>[4x]SRRTYTLTDYLKSTFRVKFYTLQWISDHEYLYKQENNILLFNAEYGNSSIFLENSTFDELGYSTNDYSVSPDRQFILFEYNYVKQWRHSYTASYDIYDLNKRQLITEERIPNNTQWITWSPVGHKLAYVWNNDIYVKNEPNLSSQRITWTGKENVIYNGVTDWVYEEEVFSAYSALWWSPNGTFLAYAQFNDTEVPLIEYSFYSDESLQYPKTVRIPYPKAGAENPTVKFFVVDTRTLSPNASVTSYQIVPPASVLIGDHYLCGVTWVTEERISLQWIRRAQNYSIIDICDYDESTGRWISSVARQHIEISTTGWV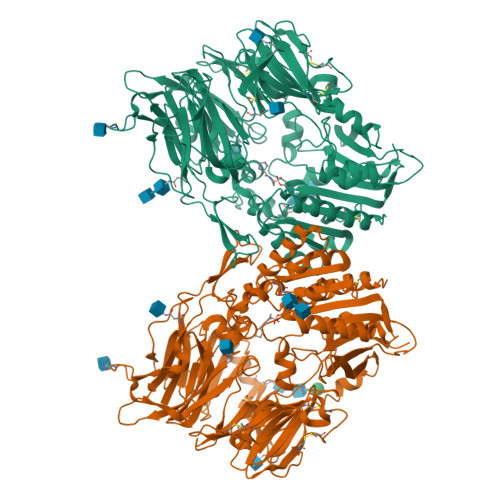GRFRPAEPHFTSDGNSFYKIISNEEGYKHICHFQTDKSNCTFITKGAWEVIGIEALTSDYLYYISNEHKGMPGGRNLYRIQLNDYTKVTCLSCELNPERCQYYSASFSNKAKYYQLRCFGPGLPLYTLHSSSSDKELRVLEDNSALDKMLQDVQMPSKKLDVINLHGTKFWYQMILPPHFDKSKKYPLLIEVYAGPCSQKVDTVFRLSWATYLASTENIIVASFDGRGSGYQGDKIMHAINRRLGTFEVEDQIEATRQFSKMGFVDDKRIAIWGWSYGGYVTSMVLGAGSGVFKCGIAVAPVSKWEYYDSVYTERYMGLPTPEDNLDYYRNSTVMSRAENFKQVEYLLIHGTADDNVHFQQSAQLSKALVDAGVDFQTMWYTDEDHGIASNMAHQHIYTHMSHFLKQCFSLP>MRSRRVDVMDVMNRLILAMDLMNRDDALRVTGEVREYIDTVKIGYPLVLSEGMDIIAEFRKRFGCRIIADFKVADIPETNEKICRAT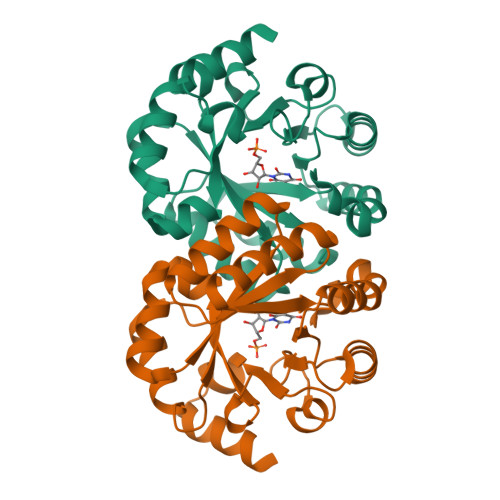FKAGADAIIVHGFPGADSVRACLNVAEEMGREVFLLTEMSHPGAEMFIQGAADEIARMGVDLGVKNYVGPSTRPERLSRLREIIGQDSFLISPGAGAQGGDPGETLRFADAAIVGRSIYLADNPAAAAAGIIESIKDLLNP[2x]bis(2-hydroxyethyl) benzene-1,4-dicarboxylate | C12 H14 O6 | 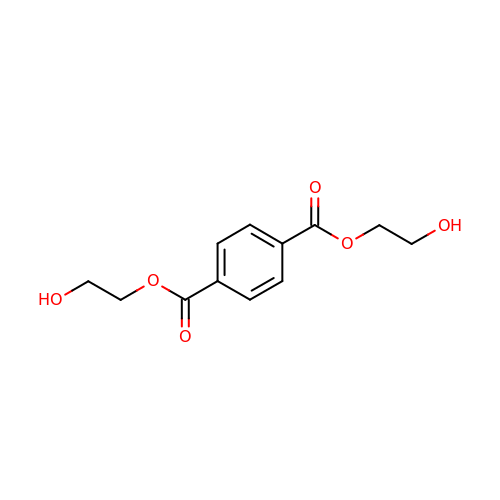QPKOBORKPHRBPS-UHFFFAOYSA-N> GASCSGGDKSKAPVVSTADIENAAEVIKYYNTSLGVLKDMVKEKDVNAVLDYMEQKGKTPALSAIVPPAVVSKDSAIVLNPGNCFNEE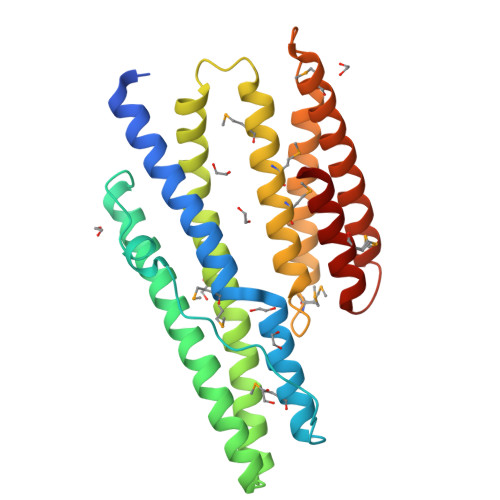TRRNLKQNYTGLFQARTEFYANFDTYLSYLKKKDVTNAKKLLDVNYQLSTQMSEYKQNIFDILSPFTEQAELVLLVDNPLKAQIMSVRKMSSTMQSILNLYARKHRMDGPRIDLKVAELTKQLDAAKKLPVVNGHEGEMKSYQAFLSQVETFIKQVKKVREKGEYSDADYDMLTSAFETSII>KVWG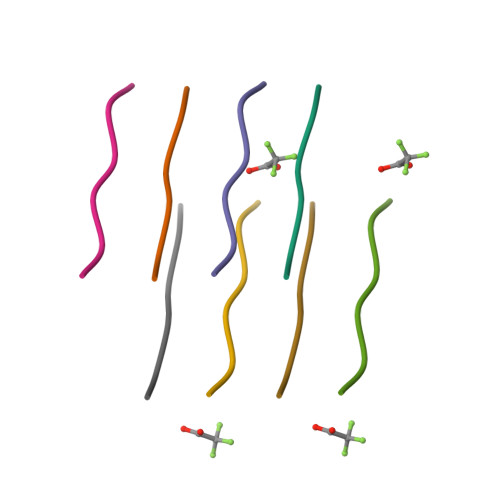SI[2x]>[2x]MNEMLKH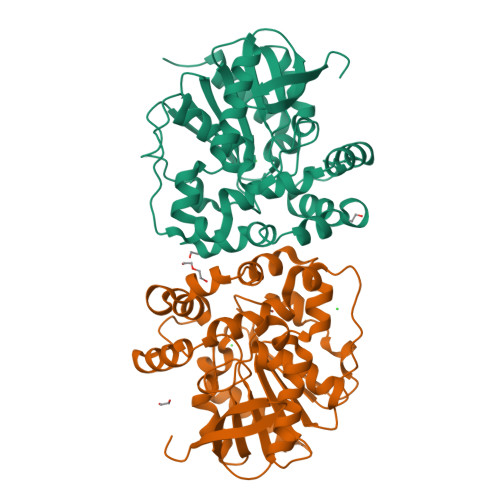EYVKVNGIKMHYVTQGKGKLLLLLHGFPDFWYVWRFQIPALAKHFRVVAPDLRGYNETDKPEGVENYRLDLLAKDILGLIKALGEEHAVVVGHDWGGIISWTLTAFNPQAVEKLVILNAPHPKAYMTRTKNSLRQLQKSWYVFFFQVANIPEKILSRNEFAFLKNMLIQSFVRRDLLTEEDLRIYVDAWSKSGALTSALNYYRANLNPDIIFSEKTVVFPKIKVPTLVIWGEKDVAISKDLIVNMEDFIEAPYSIKYFPECGHWVQLEEPELVRKHIEEFILKSDIHHHHHH> MAGQQGRELQTVVREMENFME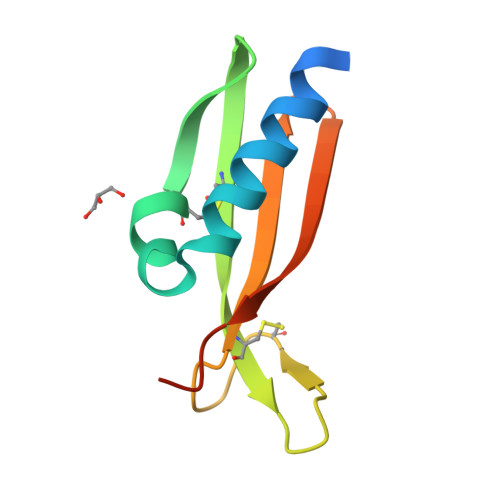RLRQDPQGIPALCNGALALGGKQGTCTAIPCNVAQDGGLACPTAGDVRAFQVVLRVEEKRLETVVYRPLEHHHHHH> HHHHVKLSVVEQAPVVEGLTPAHSLQHSIELARLADRLGYERFWVAEHHAEIFNAVPAPEILIARIAAETSGIRVGSGGVLLSLYSPLKVAEVFRTLHALYPDRIDLGIGRANRVKLPVFAALRDDTAGKEPSSD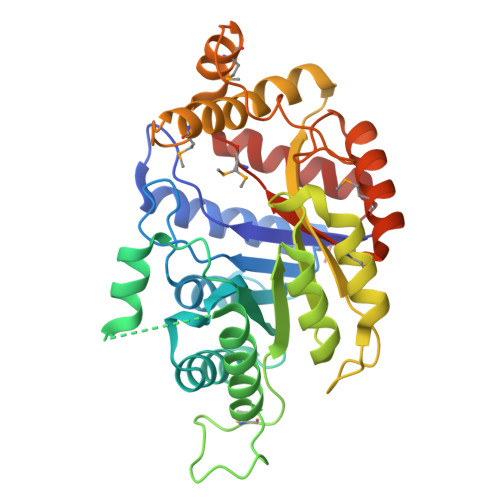DLWRRLEQLRAYLDPDSGLPFTVSPRMPGGPALWLLGASVSSAEAAARLGLPYAYAHFITPQFTREAMDTYRAAFVPGPDTPSPRPILSVVVCCAETDAEAQRVYATHRLFHRRMSQGDVRLLPPADLAVAEMDKPGPDPLAEESFEWPRYVVGSPDRVRDQLTKMADATGAEELGVVSMIHDQRDRLRSYRLLAEAFELTPR Here we characterize a metal-dependent, bifunctional isoprenyl diphosphate synthase from the leaf beetle Phaedon cochleariae by structural and functional analyses. Isoprenyl diphosphate synthase in P. cochleariae (PcIDS1, EC 2.5.1.1) produces FPP in the presence of Mg2+, but preferably forms GPP when exposed to the heavy metal ions (HMIs) Co2+ or Mn2+. Inter- and intramolecular cooperative effects in the homodimer strongly depend on the provided metal ions and regulate the biosynthetic flux of terpene precursors to either biological defence or physiological development. Strikingly, a unique chain length determination domain adapts to form geranyl or farnesyl pyrophosphate by altering enzyme symmetry and ligand affinity between both subunits.

In this complex, ZOLAl displaces GPPAl, and the structural rearrangements prevent formation of the allosteric specificity pocket. However, GPP still binds to the HAl site by inverting its PP moiety and exposing the prenyl unit towards the protein surface. Taken together, GPPAllo represents a competitive inhibitor to IPPHAl that stabilizes the open state in the presence of HMIs.

> GSFSKEESREFMAIFPDIVRDLTDAGRHTDIPEVTKRFAKVLQYNVPTGKKTRGLSTVIAYKMLEKPENLTPENVRLAGILGWCVELLQASLLIMDDLMDRSETRRGQPCWYRQENVGFLAINDCLHVESSLYSVLRKYFSHLPCYVPIIELFHDVNFKTNMGQSLDALCMKDGRPILSQFTMKRYSSIVKYKTSYYTFQLPVSLGMYLADMYDPEQHRQAKTILMEIGEFFQIQDDFLDAFGDSQVTGKVGTDIKEGKCSWLAVVALQRSNPAQRQIMEEHYGRPEPESTQIIKNLYIELGLPATFAVYEEESFNIIRTHIHQISKGLPHDLFFKIMKKIYKRDA> GAMGIAAKREENFSAWYIDVITKAEMIEYYDVSGCYIIRPWAYYVWKCVQRFLGGKIEKLGVEDCYFPMFVSRSCLEREKDHIEGFAPEVAWVTRAGDTELEQPVAVRPTSETVMYPYYAKWIRSHRDLPVRLNMWNNVIRWEFSHPTPFIRTREFLWQEGHCAWAKAEECAKEVLEILECYASVYEQLLAVP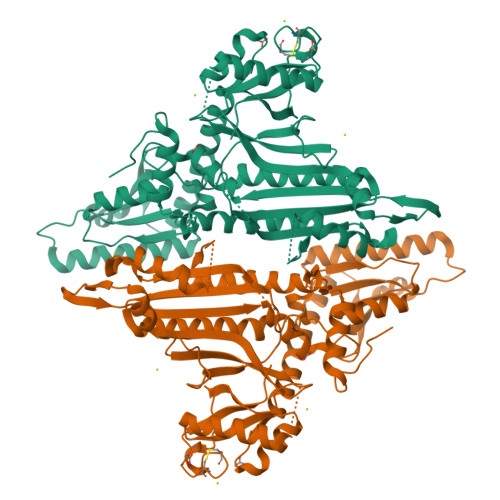VVRGRKTEKEKFAGGDYTTTVETFIEAVGRGCQGATSHNLGQNFGKMFDIRFQDPENNEQTLIPWQNSWGLSTRVIGVMIMVHGDNRGMVMPPRVASTQVIIIPVGITKDTTEEARQELLASCWRLESELCEGGVRARCDLRDNYSPGWRFNHWEVKGVPLRVELGPRELAERSLAVAVRHSGARHSVAWDAQTPAAVAALLEDVHAQMYARAKETMETHRVRVTEWTEFVPTLNRKCLILAPWCGAMECENQVKKDSAEESKVAQAQETREDARAPSMGAKTLCIPFEQPEEPAEGHECICKGCTKPATTWVLFGRSY2-deoxy-3-O-[(3R)-3-hydroxytetradecanoyl]-2-{[(3R)-3-hydroxytetradecanoyl]amino}-4-O-phosphono-beta-D-glucopyranose 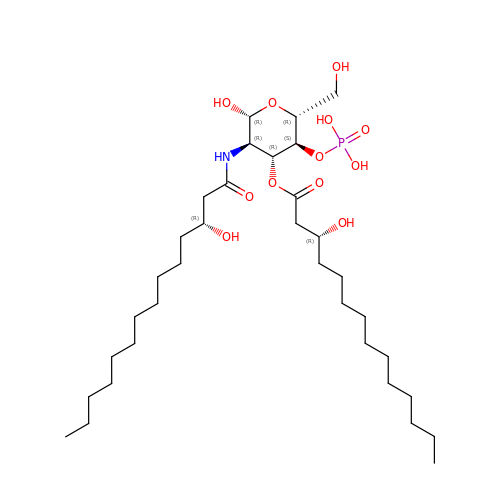| C34 H66 N O12 P | AJRPJFBMHCTNGK-XQJZMFRCSA-N> GSNNVLPTWSLDSNGEMRSRLSLSEVLDSGDLMKFAVDKTGCQFLEKAVKGSLTSYQKFQLFEQVIGRKDDFLKLSTNIFGNYLVQSVIGISLATNDDGYTKRQEKLKNFISSQMTDMCLDKFACRVIQSSLQNMDLSLACKLVQALPRDARLIAICVDQNANHVIQKVVAVIPLKNWEFIVDFVATPEHLRQICSDKYGAYVVQTIIEKLTADSMNVDLTSAAQNLRERALQRLMTSVTNRCQELATNEYANYIIQHIVSNDDLAVYRECIIEKCLMRNLLSLSQEKFASHVVEKAFLHAPLELLAEMMDEIFDGYIPHPDTGKDALDIMMFHQFGNYVVQCMLTICCDAVSGRRQTKEGGYDHAISFQDWLKKLHSRVTKERHRLS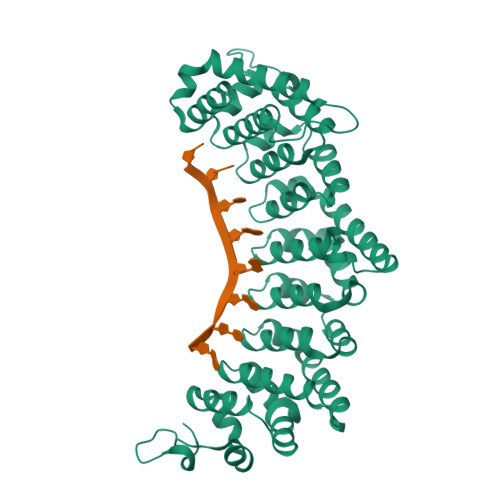RFSSGKKMIETLANLRSTHPIYELQ> MPVHGVIYYSSPSMATFLSPAQDN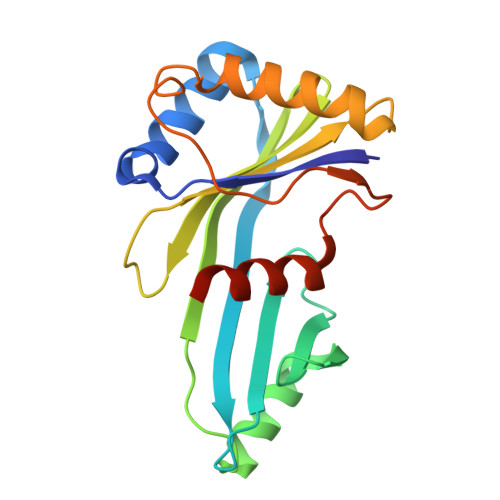LVRTYFAQHLKKWVVQYKLYRNAVTPKTLEFLKQNINPSMLACVDEATMIDAEPELEDIIVRTKLWNFRQSFTIEGSIYEVGSFKVAIANVLQKSVWKGILFHVTYDGTESVDLARPIIQEFFLKCFLQNNKSVTPVYESFFNQPRHSLDSKLLLQLFKQRIDTVSQRT> MGSSHHHHHHSQDPNSMSAVQPFIRTNIGSTLRIIEEPQRDVYWIHMHADLAINPGRACFSTRLVDDITGYQTNLGQRLNTAGVLAPHVVLASDSDVFNLGGDLALFCQLIREGDRARLLDYAQRCVRGVHAFHVGLGARAHSIALVQGNALGGGFEAALSCHTIIAEEGVMMGLPEVLFDLFPGMGAYSFMCQRISAHLAQKIMLEGNLYSAEQLLGMGLVDRVVPRGQGVAAVEQVIRESKRTPHAWAAMQQVREMTTAVPLEEMM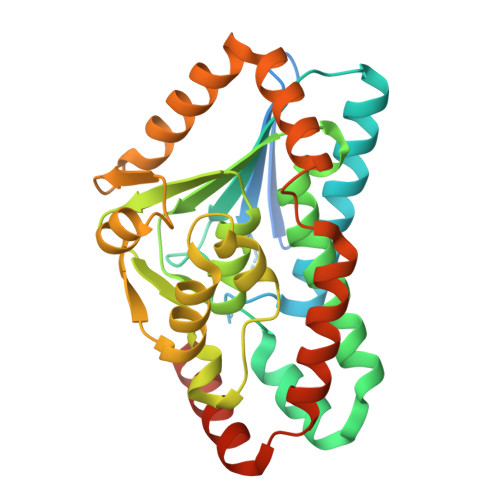RITEIWVDTAMQLGEKSLRTMDRLVRAQSRRSGLDAG> MRALLPYLALYKRHKWMLSLGIVLAIVTLLASIGLLTLSGWFLSASAVAGVAGLYSFNYMLPAAGVRGAAITRTAGRYFERLVSHDATFRVLQHLRIYTFSKLLPLSPAGLARYRQGELLNRVVADVDTLDHLYLRVISPLVGAFVVIMVVTIGLSFLDFTLAFTLGGIMLLTLFLMPPLFYRAGKSTGQNLTHLRGQYRQQLTAWLQGQAELTIFGASDRYRTQLENTEIQWLEAQRRQSELTALSQAIMLLIGALAVILMLWMASGGVGGNAQPGALIALFVFCALAAFEALAPVTGAFQHLGQVIASAVRITDLTDQKPEVTFPDTQTRVADRVSLTLRDVQFTYPEQSQQALKGISLQVNAGEHIAILGRTGCGKSTLLQLLTRAWDPQQGEILLNDSPIASLNEAALRQTISVVPQRVHLFSATLRDNLLLASPGSSDEALSEILRRVGLEKLLEDAGLNSWLGEGGRQLSGGELRRLAIARALLHDAPLVLLDEPTEGLDATTESQILELLAEMMREKTVLMVTHRLRGLSRFQQIIVMDNGQIIEQGTHAELLARQGRYYQFKQGLHLGGIKAFDYKDDDDK;> MNKSRQKELTRWLKQQSVISQRWLNISRLLGFVSGILIIAQAWFMARILQHMIMENIPREALLLPFTLLVLTFVLRAWVVWLRERVGYHAGQHIRFAIRRQVLDRLQQAGPAWIQGKPAGSWATLVLEQIDDMHDYYARYLPQMALAVSVPLLIVVAIFPSNWAAALILLGTAPLIPLFMALVGMGAADANRRNFLALARLSGHFLDRLRGMETLRIFGRGEAEIESIRSASEDFRQRTMEVLRLAFLSSGILEFFTSLSIALVAVYFGFSYLGELDFGHYDTGVTLAAGFLALILAPEFFQPLRDLGTFYHAKAQAVGAADSLKTFMETPLAHPQRGEAELALTDPLTIEAEDLFITSPEGKTLAGPLNFTLPAGQRAVLVGRSGSGKSSLLNALSGFLSYQGSLRINGIELRDLSPESWRKHLSWVGQNPQLPAATLRDNVLLARPDASEQELQAALDNAWVSEFLPLLPQGVDTPVGDQAARLSVGQAQRVAVARALLNPCSLLLLDEPAASLDAHSEQRVMEALNAASLRQTTLMVTHQLEDLADWDVIWVMQDGRIIEQGRYAELSVAGGPFATLLAHRQEEI

CydDC is a prokaryotic ATP-binding cassette (ABC) transporter required for heme assembling in respiratory cytochrome bd oxidase, a promising target for drug discovery. In our structures, CydC and CydD form a heterodimer with each subunit composed of one transmembrane domain (TMD) and one nucleotide-binding domain (NBD). TM4 and TM5 of one subunit associate with TM1-3 and TM6 of another to form a helix bundle in a “domain swapping” manner. The overall fold of CydDC belongs to the type IV family of ABC transporters, commonly known as exporters.

In the Cryo-EM map of heme-loading EcCydDC, we observed a clear density of heme molecule enclosed by TM4–6 of EcCydD and TM2–3 of EcCydC. However, the location of heme is not in the middle of TM region or in the central cavity. Crucially, two axial His residues, His85 in TM2C and His312 at the bending point of TM6D, coordinate axially to the central iron atom of the heme from opposite sides. Such a binding pattern, is commonly observed in many heme-associated enzymes, but never seen in other heme transporters. The tetrapyrrole group in heme is further immobilized by many surrounding residues. In the heme-loading structure, the two axial His residues are 4.8 Å away from each other, which is perfect to clamp the iron ion. In the heme-loading structure of EcCydDC, the corresponding distance is shortened to 13.8 Å. There is still a hole left, leading to the heme binding site. However, it is not large enough to allow the heme to pass through. Interestingly, the long EH of EcCydD protrudes and interacts with TM4D in the heme-loading structure.>FDHCFKKSSDGFLYCEGTKVEDIMESVERRPFYLYSKPQITRNLEAYKEALEGVSSVIGYAIKANNNLKILEHLRSLGCGAVLVSGNELRLALRAGFDPTKCIFNGNGKSLEDLVLAAQEGVFVNVDSEFDLNNIVEASRISGKQVNVLLRINPDVDPQVHPYVATGNKNSKFGIRNEKLQWFLDQVKAHPKELKLVGAHCHLGSTITKVDIFRDAAVLMIEYIDEIRRQGFEVSYLNIGGGLGIDYYHAGAVLPTPMDLINTVRELVLSRDLNLIIEPGRSLIANTCCFVNHVTGVKTNGTKNFIVIDGSMAELIRPSLYDAYQHIELVSPPPAEAEVTKFDVVGPVCESAD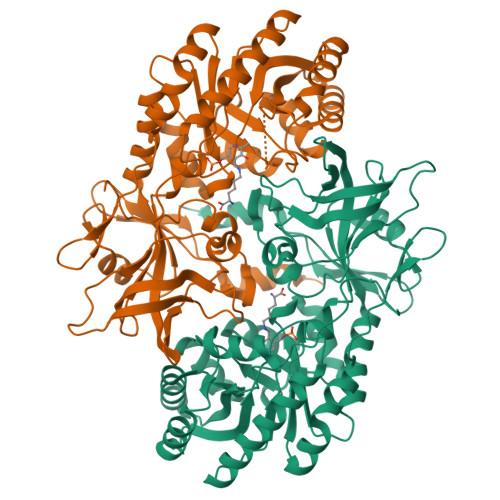FLGKDRELPTPPQGAGLVVHDAGAYCMSMASTYNLKMRPPEYWVEEDGSITKIRHAETFDDHLRFFEGL[2x]>[2x]ALGVVGVLESYIGSINNITKQSACVAMSKLLTELNSDDIKKLRDNEELNSPKIRVYNTVISYIESNRKNNKQTIHLLKRLPADVLKKTIKNTLDIHKSITINNPKELTVSDTN

The M2–1 transcription antiterminator factor is a basic protein of 194 amino acids that exists as a stable tetramer in solution and is essential for the complete sequential transcription of mRNAs in HRSV. It harbours four distinct regions: an N-terminal zinc-binding domain (ZBD; residues 7–25), an α-helical tetramer­ization domain (TD; residues 32–49), an RNA-binding core domain (RBD; residues 69–172) and a C-terminal unstructured region (residues 173–194). A crystal structure of the tetrameric M2–1 assembly and an NMR structure of the monomeric M2–1 RBD (residues 58–177; Blondot et al., 2012) have been determined. M2–1 oligomerization is primarily driven by a central tetramerization α-helix and is also stabilized by contacts between the zinc-binding domain and the core of an adjacent monomer. Given the relevance and uniqueness of this viral transcription antiterminator, we set out to investigate its RNA-binding domain (residues 73–194) using X-ray crystallography and folding thermodynamics.

The HRSV M2–1 RBD crystallized with two molecules in the asymmetric unit. The structures from both crystal forms are virtually identical in the core region (residues 58–177), with a root-mean-square deviation (r.m.s.d. on Cα atoms) of 0.3 Å. The structure of the monomeric domain is superimposable with that of the tetramer, but uncovers additional structured residues at the C-terminus that have not been observed previously. A notable exception is the C-terminal region (residues 178–185), which could be clearly modelled in one monomer in the P3221 crystal form. In the tetrameric HRSV M2–1 crystal structure this region was disordered and thus not visible. The C-terminal tail observed in our P3221 model could be extended in solution and would therefore explain the lack of globularity in our SAXS model. Electron density for this region has not been observed in previous crystal structures. On the other hand, the crystal structures presented here strongly suggest that the carboxy-terminal region of the protein would be unstructured in the closed conformation present in the RNA-free tetramer and folds upon the helical cleft corresponding to the ZBD-binding region in the RBD.> SWQTYVDTNLVGTGAVTQAAIIGHDGNTWATSAGFAVSPANGAALANAFKDATAIRSNGFELAGTRYVTIRADDRSVYGKKGSA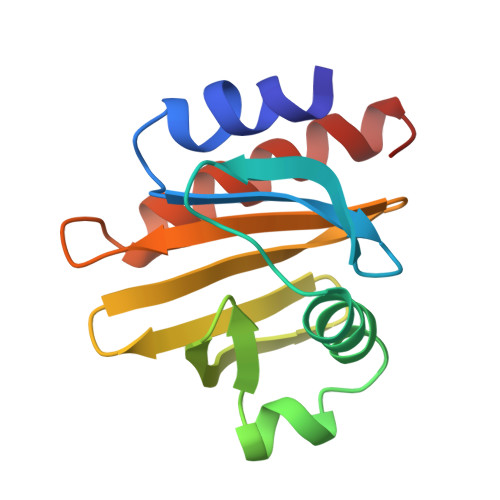GVITVKTSKAILIGVYNEKIQPGTAANVVEKLADYLIGQGF> YTAVPSCIPS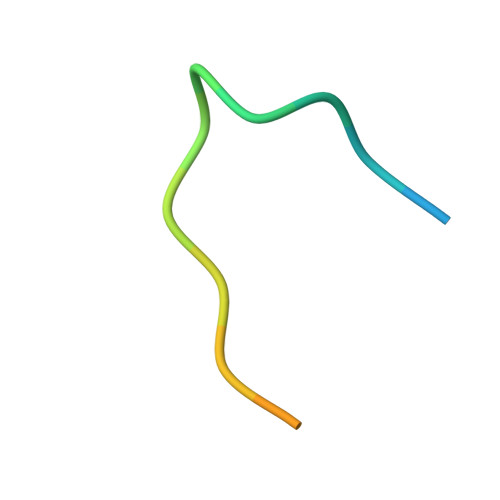RASILTGM> MMA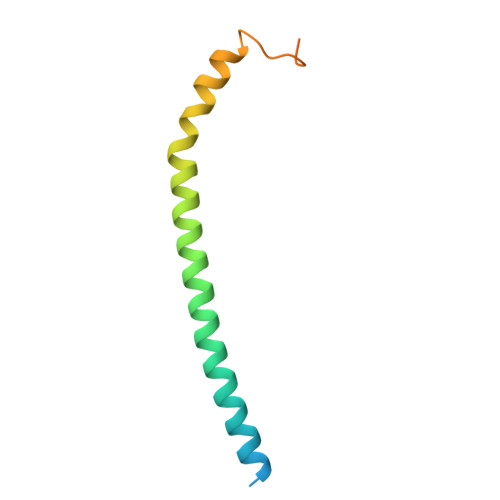STSNDEEKLISTTDKYFIEQRNIVLQEINETMNSILNGLNGLNISLESSIAVGREFQSVSDLWKTLYDGLESLSDEAPIDEQPTLSQSKTK> GAMGSEQRASLDSEESESPPQENSCLDPPDRDPNCKPPPVKPHIFTTRSRTRLFGKGDSEEASPLDCPYEEGGLASCPIITVSSVLTIQRPGDGPASVRPSSQDSVSAGEKPPRLYDRRSIFDAVAQSNCQELESLL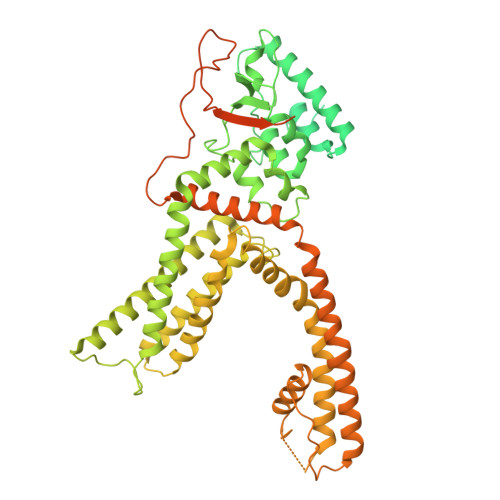PFLQRSKKRLTDSEFKDPETGKTCLLKAMLNLHNGQNDTIALLLDVARKTDSLKQFVNASYTDSYYKGQTALHIAIERRNMTLVTLLVENGADVQAAANGDFFKKTKGRPGFYFGELPLSLAACTNQLAIVKFLLQNSWQPADISARDSVGNTVLHALVEVADNTVDNTKFVTSMYNEILILGAKLHPTLKLEEITNRKGLTPLALAASSGKIGVLAYILQREIHEPECRHLSRKFTEWAYGPVHSSLYDLSCIDTCEKNSVLEVIAYSSSETPNRHDMLLVEPLNRLLQDKWDRFVKRIFYFNFFVYCLYMIIFTAAAYYRPVEGLPPYKLKNTVGDYFRVTGEILSVSGGVYFFFRGIQYFLQRRPSLKSLFVDSYSEILFFVQSLFMLVSVVLYFSQRKEYVASMVFSLAMGWTNMLYYTRGFQQMGIYAVMIEKMILRDLCRFMFVYLVFLFGFSTAVVTLIEDGKNNSLPMESTPHKCRGSACKPGNSYNSLYSTCLELFKFTIGMGDLEFTENYDFKAVFIILLLAYVILTYILLLNMLIALMGETVNKIAQESKNIWKLQRAITILDTEKSFLKCMRKAFRSGKLLQVGFTPDGKDDYRWCFRVDEVNWTTWNTNVGIINEDPGNCEGVKRTLSFSLRSGRVSGRNWKNFALVPLLRDASTRDRHATQQEEVQLKHYTGSLKPEDAEVFKDSMVPGEK>[3x]MDSKEVLVHVKNLEKNKSN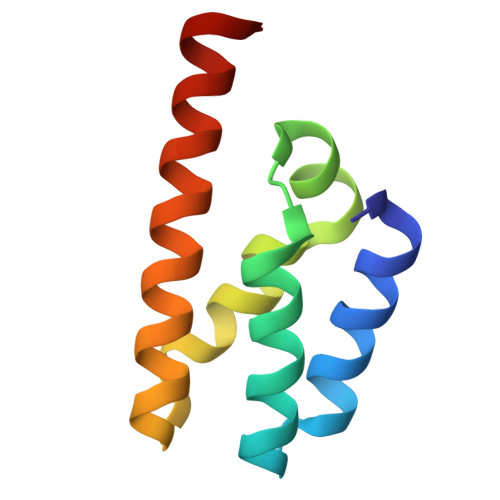DAAVLEILHVLDKEFVPTEKLLRETKVGVEVNKFKKSTNVEISKLVKKMISSWKAQLNLENLYFQG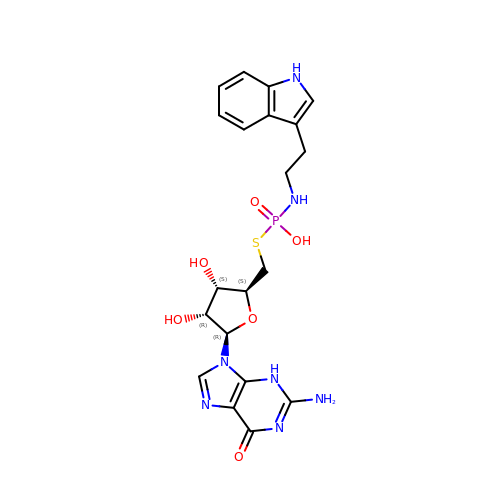5'-S-[(S)-hydroxy{[2-(1H-indol-3-yl)ethyl]amino}phosphoryl]-5'-thioguanosine | C20 H24 N7 O6 P S | WJQUHDQKVRSGDO-NVQRDWNXSA-N ACETIC ACID N-[2-CHLORO-5-[6-ETHYL-2,4-DIAMINO-PYRIMID-5-YL]-PHENYL]-[BENZYL-TRIAZEN-3-YL]ETHYL ESTER | C23 H26 Cl N7 O2 | 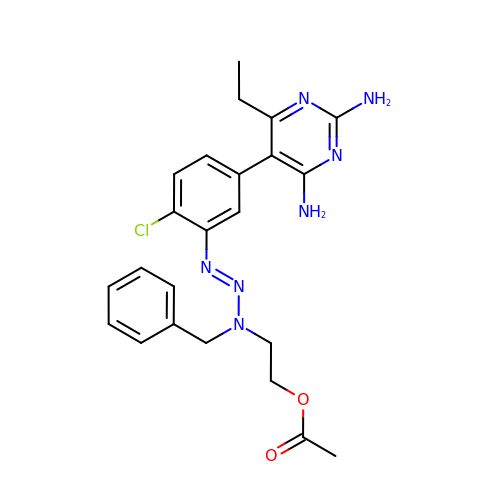QKBISNUGIKKCIM-QVIHXGFCSA-N> GPGS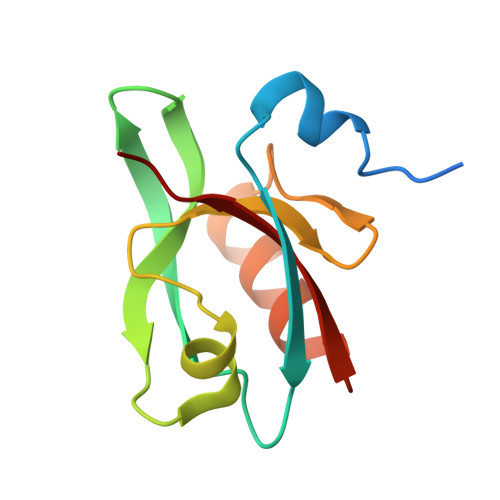KKFPTASDETKFIFDQFPKARTVQVRKEGFLGIMVIYGKHAEVGSGIFISDLREGSNAELAGVKVGDMLLAVNQDVTLESNYDDATGLLKRAEGVVTMILLTLK1-(diphenylmethyl)azetidin-3-ol | C16 H17 N O | 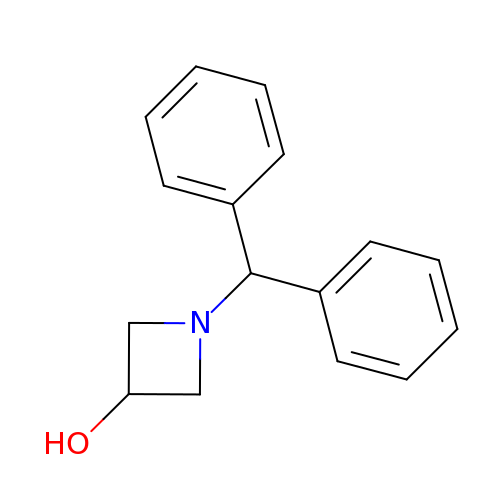MMAJXKGUZYDTHV-UHFFFAOYSA-N>[4x]MQFRSIIRIVGLLLALFSVTMLAPALVALLYRDGAGVPFVTTFFVLLFCGAMCWFPNRRHKHELKSRDGFLIVVLFWTVLGSAGSLPFLIADNPNISVTDAFFESFSALTTTGATVIVGLDELPKAILFYRQFLQWFGGMGIIVLAVAILPVLGIGGMQLYRAEIPGPVKDTKMTPRIAETAKALWYIYLSLTIACAVAFWLAGMTPFDAISHSFSTIAIGGFSTHDASMGYFDSYAINLITVVFLLISACNFTLHFAAFASGGVHPKYYWKDPEFRAFIFIQVLLFLVCFLLLLKHHSYTSPYDAFDQALFQTVSISTTAGFTTTGFADWPLFLPVLLLFSSFIGGCAGSTGGGMKVIRILLLTLQGARELKRLVHPRAVYTIKVGGSALPQRVVDAVWGFFSAYALVFVVCMLGLIATGMDELSAFSAVAATLNNLGPGLGEVALHFGDVNDKAKWVLIVSMLFGRLEIFTLLILLTPTFWRS;>MKIIILGAGQVGGTLAENLVGENNDITIVDNNADRLRELQDKYDLRVVNGHASHPDVLHEAGAQDADMLVAVTNTDETNMAACQVAFTLFNTPNRVARIRSPEYLAEKEALFKSGAIPVDHLIAPEELVTSYIERLIQYPGALQVVSFAEQKVSLVAVKAYYGGPLVGNALSALREHMPHIDTRVAAIFRQGRPIRPQGTTIIEADDEVFFVAASNHIRSVMSELQRLEKPYRRIMIVGGGNIGASLAKRLEQTYSVKLIERDYQRAEKLSEQLENTIVFCGDAADQELLTEENIDQVDVFIALTNEDETNIMSAMLAKRMGAKKVMVLIQRGAYVDLVQGGVIDVAISPQQATISALLTHVRRADIVNVSSLRRGAAEAIEAVAHGDETTSKVVGRAIGDIKLPPGTTIGAVVRGEEVLIAHDRTVIEQDDHVVMFLVDKKYVPDVEALFQPSPFFL[4x]

TrkH, KtrB, and more distantly related KdpA belong to the superfamily of K+ transporters (SKTs) that are found in bacteria, fungi, and plants. TrkH or KtrB proteins assemble with their respective cytosolic partner proteins TrkA or KtrA to form a stable complex. To better understand the mechanism by which the Trk system functions, we determined the structures of TrkH-TrkA complex from V. parahaemalyticus in the presence of ADP (TrkHA-ADP), ATP (TrkHA-ATP), or ATPγS (TrkHA-ATPγS).

The structure of TrkHA-ATP was solved by cryo-electron microscopy (cryo-EM) to an overall resolution of 3.0 Å. The TrkHA protein was frozen to the cryo-EM grids in the presence of 10 mM ATP. Interestingly, TrkH is in a partially open conformation and the dimer interface is also different from that of TrkHA-ADP. First, in the presence of ATP, the N2-N2 interface is lost, and as a result, TrkA tetramer becomes two dimers. Second, the HN1 interface is no longer present. In the presence of ATP, the N2 domain has a rotation of 36° relative to the N1 domain when compared to the structure of a TrkA protomer in the presence of ADP. In the TrkHA-ATP structure, the tetramer-to-dimer conversion in TrkA moves the N1 domain almost 13 Å away from TrkH. In contrast, TrkH in the TrkHA-ATP is in a partially open state and the ion permeation pathway expands to more than 2.1 Å in radius below the selectivity filter. It seems that opening of the ion permeation pathway comes from an expansion of pore-lining helices and the movement of the intramembrane loop towards the intracellular side. In TrkHA-ATP, the neighboring D4M1 helices form an angle of 45°, while those of TrkHA-ADP is 59°.>[4x]AAVGEAATQTKARTRSKYEIETLTGWLLKQPMAGVIDAELTIVLSSISLACKQIASLVQRAGISNLTGIQGAVNIQ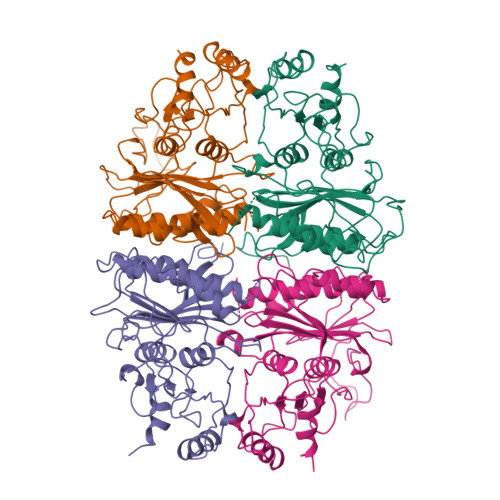GEDQKKLDVVSNEVFSSCLRSSGRTGIIASEEEDVPVAVEESYSGNYIVVFDPLDGSSNIDAAVSTGSIFGIYSPNDECIVDSDHDDESQLSAEEQRCVVNVCQPGDNLLAAGYCMYSSSVIFVLTIGKGVYAFTLDPMYGEFVLTSEKIQIPKAGKIYSFNEGNYKMWPDKLKKYMDDLKEPGESQKPYSSRYIGSLVGDFHRTLLYGGIYGYPRDAKSKNGKLRLLYECAPMSFIVEQAGGKGSDGHQRILDIQPTEIHQRVPLYIGSVEEVEKLEKYLA>[2x]MRPVFPLILSAVLFLSCFFGARQTEASASKRAIDANQIVNRMSLDEKLGQMLMPDFRNWQKEGESSPQALTKMNDEVASLVKKYQFGGIILFAENVKTTKQTVQLTDDYQKASPKIPLMLSIDQEGGIVTRLGEGTNFPGNMALGAARSRINAYQTGSIIGKELSALGINTDFSPVVDINNNPDNPVIGVRSFSSNRELTSRLGLYTMKGLQRQDIASALKHFPGHGDTDVDSHYGLPLVSHGQERLREVELYPFQKAIDAGADMVMTAHVQFPAFDDTTYKSKLDGSDILVPATLSKKVMTGLLRQEMGFNGVIVTDALNMKAIADHFGQEEAVVMAVKAGVDIALMPASVTSLKEEQKFARVIQALKEAVKNGDIPEQQINNSVERIISLKIKRGMYPARNSDSTKEKIAKAKKIVGSKQHLKAEKKLAEKAVTVLKNEQHTLPFKPKKGSRILIVAPY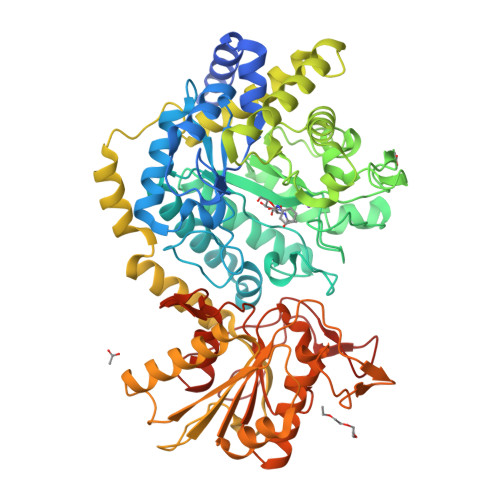EEQTASIEQTIHDLIKRKKIKPVSLSKMNFASQVFKTEHEKQVKEADYIITGSYVVKNDPVVNDGVIDDTISDSSKWATVFPRAVMKAALQHNKPFVLMSLRNPYDAANFEEAKALIAVYGFKGYANGRYLQPNIPAGVMAIFGQAKPKGTLPVDIPSVTKPGNTLYPLGYGLNIKTGRPL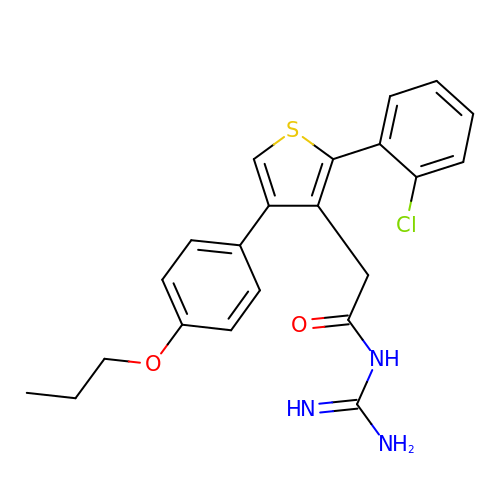N-[amino(imino)methyl]-2-[2-(2-chlorophenyl)-4-(4-propoxyphenyl)-3-thienyl]acetamide | C22 H22 Cl N3 O2 S | VZSMTBLDWPKVRW-UHFFFAOYSA-N>MSAVMATYLLHDETDIRKKAEGIALGLTIGTWTDLPALEQEQLRKHKGEVVAIEELGESERVNAYFGKRLKRAIVKIAYPTVNFSADLPALLVTTFGKLSLDGEVRLLDLEFPDEWKRQFPGPRFGIDGIRDRVGVHNRPLLMSIFKGMIGRDLAYLTSELKKQALGGVDLVKDDEILFDSELLPFEKRITEGKAALQEVYEQTGKRTLYAVNLTGKTFALKDKAKRAAELGADVLLFNVFAYGLDVLQALREDEEIAVPIMAHPAFSGAVTPSEFYGVAPSLWLGKLLRLAGADFVLFPSPYGSVALEREQALGIARALTDDQEPFARAFPVPSAGIHPGLVPLI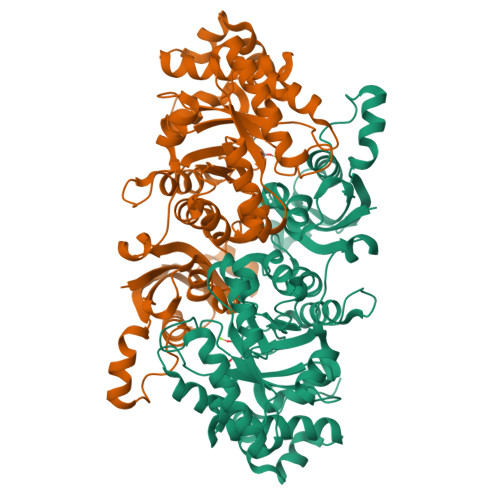IRDFGLDTIVNAGGGIHGHPDGAIGGGRAFRAAIDAVLAGRPLRAAAAENEALQKAIDRWGVVEVEA[2x]> GPLGSG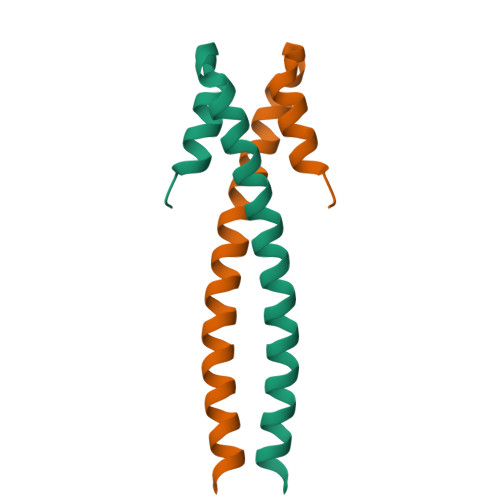VGNGDDEAAELMQQVNVLKLTVEDLEKERDFYFGKLRNIELICQENEGENDPVLQRIVDILYATDEGFVI>MDNQKGRISIALLPFLAHGHISPFFELAKQLAKRNCNVFLCSTPINLSSIKDKDSSASIKLVELHLPSSPDLPPHYHTTNGLPSHLMLPLRNAFETAGPTFSEILKTLNPDLLIYDFNPSWAPEIASSHNIPAVYFLTTAAASSSIGLHAFKNPGEKYPFPDFYDNSNIIPEPPSADNMKLLHDFIACFERSCDIILIKSFRELEGKYIDLLSTLSDKTLVPVGPLVQDPMGHNEDPKTEQIINWLDKRAESTVVFVCFGSEYFLSNEELEEVAIGLEISTVNFIWAVRLIEGEKKGILPEGFVQRVGDRGLVVEGWAPQARILGHSSTGGFVSHCGWSSIAESMKFGVPVIAMARHLDQPLNGKLAAEVGVGMEVVRDENGKYKREGIAEVIRKVVVEKSGEVIRRKARELSEKMKEKGEQEIDRAVEELVQICKKKKDEQENLYFQGHHHHHH[2x]

Pq3‐O‐UGT2, an important UDP‐dependent glycosyltransferase (UGT), catalyzes the production of Ginsenoside Rg3 and Rd by extending the glycan chain of Ginsenoside Rh2 and F2, respectively, with higher selectivity for F2. Pq3‐O‐UGT2 catalyzes glucose transfer from UDP‐Glucose (UDP‐Glc) to the C2‐OH of the C3‐glucose of Ginsenoside Rh2 and F2, respectively. In this study, we elucidated the crystal structures of both apo Pq3‐O‐UGT2 and its complexes with Ginsenoside Rh2 and F2, revealing the acceptor recognition mechanisms of Pq3‐O‐UGT2. The NTD contains a seven‐stranded parallel β‐sheet sandwiched by seven helices, while the CTD comprises a 6‐stranded parallel β‐sheet flanked by 6 helices.

Compared to the apo structure, the structure of Pq3‐O‐UGT2 with Rh2 was better resolved, particularly in the Nα5‐Nα6 and Cβ2‐Cβ3 loops, indicating reduced spatial conflict during crystal packing in the different space group. In the complex structure, the density of Rh2 is clearly observed in the NTD of Pq3‐O‐UGT2. However, the electron density of the alkyl tail is not well‐defined, likely due to its flexibility. In the complex structure, the NTD, particularly the Nα5, Nα6, and the Nα5‐Nα6 loop shift inward, with the most substantial movement occurring at the N‐terminus of Nα6 (≈5 Å). This indicates that Pq3‐O‐UGT2 undergoes conformational changes during substrate binding, and the binding of Rh2 induces a more compact conformation. In the complex structure of Pq3‐O‐UGT2, the His20 residue forms a hydrogen bond with the 2‐OH group of the C3‐glucose of Rh2, while Asp116 forms bidentate hydrogen bonds with His20. Thus, His20 and Asp116 are proposed to form a catalytic dyad that deprotonates the C2‐OH group of Rh2. By contrast, in Pq3‐O‐UGT2, Rh2 adopts a “lying” orientation (referred to as Nα5 orientation), with its tail extending toward the Nα5 helix. The Rh2‐binding pocket of Pq3‐O‐UGT2 is composed of His20, Phe15, Phe117, Asn118, Thr139, Ser143, Ile146, Gly147, Tyr164, Leu181, Phe185, Leu358, and Leu362. Surrounding the head of Rh2, Asn118 forms a hydrogen bond with the C6‐OH group of the glucose moiety, while Phe15 engages in hydrophobic interactions with the glucose ring.> SISPAQIAEALQGRGWDAEIVTDASMAGQLVDVRPEGILKCVDGRGSDNTRMGGP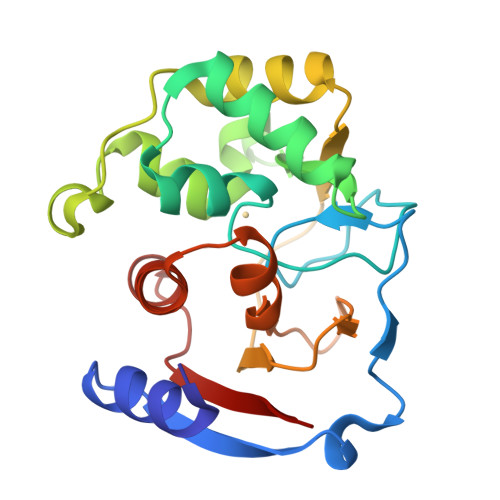KMPGGIYAIAHNRGVTSIEGLKQITKEVASKGHLPSVHGDHSSDMLGCGFFKLWVTGRFDDMGYPRPQFDADQGANAVKDAGGIIEMHHGSHTEKVVYINLLANKTLEPNENDQRFIVDGWAADKFGLDVPKFLIAAAATVEMLGGPKNAKIVVP> GMTKAREFLGTGWKFPVAAGADGAMVLSSAEEDIAESIRIILGTARGERVMRP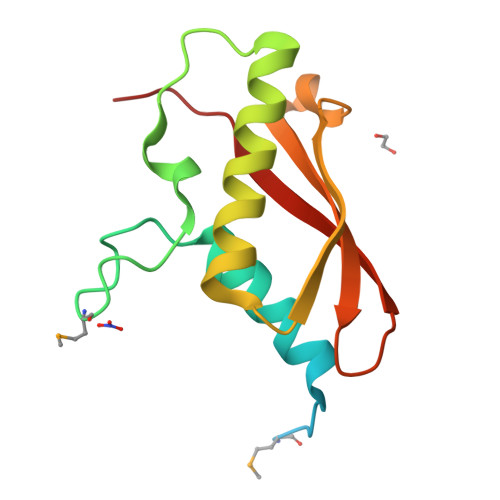DFGCGIHDRVFSVINTTTLGLIENEVKEALILWEPRIELLSVTASPREAAEGRLLIDIEYRVRSTNTRFNLVYPFYLKESA> ATPAAQASDDRYEVTQQRNPDAACLDCHKPDTEGMHGKHASVINPNNKLPVTCTNCHGQPSPQHREGVKDVMRFNEPMYKVGEQNSVCMSCHLPEQLQKAFWPHDVHVTKVACASCHSLHPQQDTMQTLSDKGRIKICVDCHSDQRTNPNFNPASV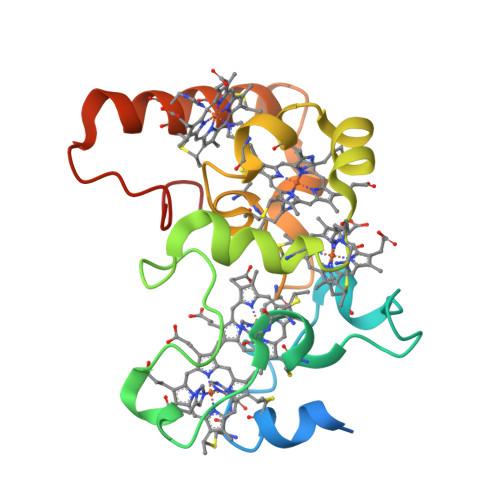PLLKEQP> MKKEVRKVRIALASPEKIRSWSYGEVEKPETINYRTLKPERDGLFDERIFGPIKDYECACGKYKRQRFEGKVCERCGVEVTRSIVRRYRMGHIELATPAAHIWFVKDVPSKIGTLLDLSATELEQVLYFNKYIVLDPKGAVLDGVPVEKRQLLTDEEYRELRYGKQETYPLPAGVDALVKDGEEVVKGQELAPGVVSRMDGVALYRFPRRVRVDYLRKERAALRIPLSAWVEKEAYRPGEVLAELSEPYLFRAEESGVVELKDLAEGHLIYLRQEEEVVARYFLPAGMTPLVVEGEIVEVGQPLAEGKGLLRLPRHMTAKEVEAEEEGDSVHLTLFLEWTEPKDYKVAPHMNVIVPEGAKVQAGEKIVAAIDPEEEVIAEAEGVVHLHEPASILVVKARVYPFEDDVEVTTGDRVAPGDVLADGGKVKSEIYGRVEVDLVRNVVRVVESYDIDARMGAEAIQELLKELDLEKLERELLEEMKHPSRARRAKARKRLEVVRAFLDSGNRPEWMILEAVPVLPPDLRPMVQVDGGRFATSDLNDLYRRLINRNNRLKKLLAQGAPEIIIRNEKRMLQEAVDAVIDNGRRGSPVTNPGSERPLRSLTDILSGKQGRFRQNLLGKRVDYSGRSVIVVGPQLKLHQCGLPKRMALELFKPFLLKKMEEKAFAPNVKAARRMLERQRDIKDEVWDALEEVIHGKVVLLNRAPTLHRLGIQAFQPVLVEGQSIQLHPLVCEAFNADFDGDQMAVHVPLSSFAQAEARIQMLSAHNLLSPASGEPLAKPSRDIILGLYYITQVRKEKKGAGMAFATPEEALAAYERGEVALNAPIVVAGRETSVGRLKFVFANPDEALLAVAHGLLDLQDVVTVRYLGRRLETSPGRILFARIVGEAVGDEKVAQELIQMDVPQEKNSLKDLVYQAFLRLGMEKTARLLDALKYYGFTLSTTSGITIGIDDAVIPEEKQRYLEEADRKLRQIEQAYEMGFLTDRERYDQVIQLWTETTEKVTQAVFKNFEENYPFNPLYVMAQSGARGNPQQIRQLCGMRGLMQKPSGETFEVPVRSSFREGLTVLEYFISSHGARKGGADTALRTADSGYLTRKLVDVAHEIVVREADCGTTNYISVPLFQMDEVTRTLRLRKRSDIESGLYGRVLAREVEALGRRLEEGRYLSLEDVHFLIKAAEAGEVREVPVRSPLTCQTRYGVCQKCYGYDLSMARPVSIGEAVGVVAAESIGEPGTQLTMRTFHTGGVAVGTDIT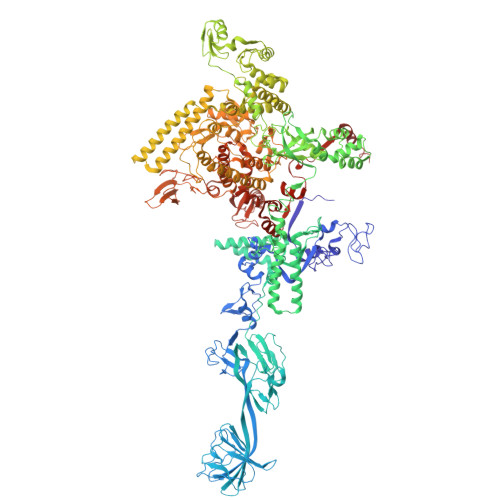QGLPRVIELFEARRPKAKAVISEIDGVVRIEEGEDRLSVFVESEGFSKEYKLPKDARLLVKDGDYVEAGQPLTRGAIDPHQLLEAKGPEAVERYLVDEIQKVYRAQGVKLHDKHIEIVVRQMLKYVEVTDPGDSRLLEGQVLEKWDVEALNERLIAEGKVPVAWKPLLMGVTKSALSTKSWLSAASFQNTTHVLTEAAIAGKKDELIGLKENVILGRLIPAGTGSDFVRFTQVVDQRTLKAIEEARKEAVEAKEKEAPRRPVRREQPGKGL> GSSGSSGMANERMNLMNMAKLSIKGLIESALNLGRTLDSDYAPLQQFFVVMEHCLKHGLKAKKTFLGQNKSFWGPLELVEKLVPEAAEITASVKDLPGLKTPV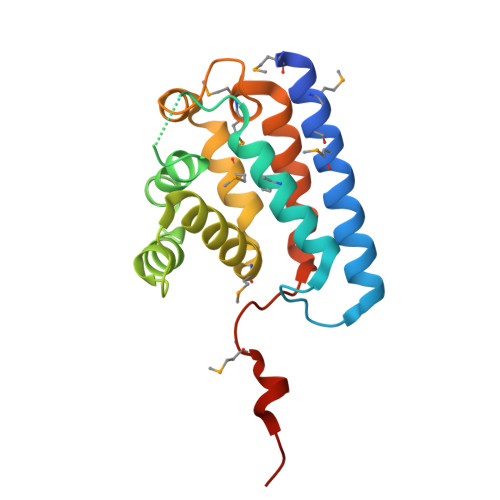GRGRAWLRLALMQKKLSEYMKALINKKELLSEFYEVNALMMEEEGAIIAGLLVGLNVIDANFCMKGEDLDSQVGVID>GSHMASMTGGQQMGRGSMKFSFELAVNTKKEDAWTYYSQVNQWFVWEGDLEQISLEGEFTTGQKGKMKMEDMPELAFTLVEVRENQCFSDLTATPFGNVLFEHEILENPDGTISLRHSVSLTDSDTTEEALAFLKQIFADVPESVGK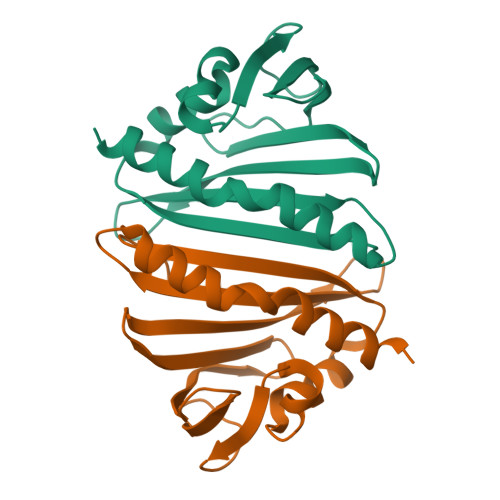LKQILETV[2x]MOSC proteins play a key role in the Moco-dependent reduction of N-hydroxylated mutagens or prodrugs as a final electron transfer enzyme in the nitrogen-reducing system. To provide insights into the catalytic mechanism of MOSC enzymes, we report two crystal structures of YiiM, one from Gram-positive Geobacillus stearothermophilus (gsYiiM) and the other from Gram-negative E. coli (ecYiiM). Based on the comparative analyses of structural and biophysical data, we present the common and distinct features of YiiM enzymes and propose the putative catalytic site that is located at a reactive invariant cysteine residue. Sequences corresponding to the β-barrel and N-α-bundle modules of YiiM are conserved in MOSC family members, suggesting that the two modules form the canonical structure of the MOSC domain.

Although the crystal structure of the TP1000-expressed ecYiiM protein was solved by molecular replacement and refined to 2.85 Å resolution, the electron density for Moco was not visible and instead a phosphate ion was identified. Interestingly, in the ecYiiMPi structure, a phosphate ion was found in the cavity of ecYiiM near the invariant cysteine residue, C120. The phosphate ion in the ecYiiMPi structure appeared to be captured from crystallization solution containing ammonium dihydrogen phosphate. The phosphate ion in the ecYiiMPi structure is stabilized by multiple hydrogen bonds with the side chains of cavity residues (Q115, S118, S200, and W201) and partially fills the cavity, leaving space for the remaining atoms of the Moco molecule in the putative catalytic site. However, the phosphate ion in the cavity serves as a guide to locate a Moco molecule in the YiiM structure because Moco contains a phosphate group at one end. The ecYiiMPi and apo-ecYiiM structures are essentially identical, with root-mean-square deviation (RMSD) values of 0.35–0.47 Å. ecYiiM exhibits a similar overall structure to gsYiiM but with significant local structural differences (RMSD 1.20–1.24 Å). ecYiiM possesses shorter β1 and β2 strands than gsYiiM. Moreover, ecYiiM contains an additional β-strand (β3s), which functions as a lid on the β-barrel along with the β3 and β9 strands. ecYiiM is also characterized by an additional C-terminal α-helix, α7, which folds back to the N-α-bundle. Consistently, the asymmetric unit of the ecYiiMPi crystal contained two ecYiiM chains, which are related by non-crystallographic two-fold symmetry. In each interface, the α5 and α6 helices of the C-α-bundle from one subunit make contacts with one side (β8′-β7′-β6′-β10′) of the β-barrel from the other subunit.

>GSAKDPMRYPVDVYTGKIQAYPEGKPSAIAKIQVDGELMLTELGLEGDEQAEKKVHGGPDRALCHYPREHYLYWAREFPEQAELFVAPAFGENLSTDGLTESNVYMGDIFRWGEALIQVSQPRSPCYKLNYHFDISDIAQLMQNTGKVGWLYSVIAPGKVSADAPLELVSRVSDVTVQEAAAIAWHMPFDDDQYHRLLSAAGLSKSWTRTMQKRRLSGKIEDFSRRLWGK[2x]>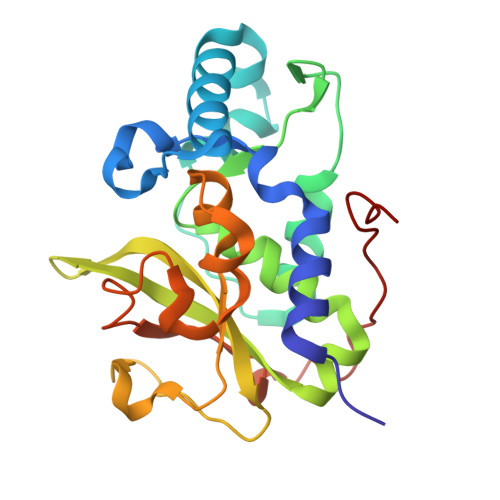 GMAIAPQQIQERLKQEQYQKFVVADIGNFPHCLAQTPEGIASGQRYQKYSTNSLSRTPPFSQWGAPQLLTPKSAQEYIKFAQQRNKKSSFKIDGEAVRVSECSNFAYHSAGVLLDDPQIRTQYDVAVIGSMHSNGRYLHNITLLVPKGSRLPQPPEQLTAEVFPIGTLIVDPWAVGMGHPPEQALAIPKEQFAYNRSLFPATVNYQSALDESLTSTRTGQLTPYTGTPS> SSQQVWKLVIITEEILLKKVSKIIKEAGASGYTVLAAAGEGSRNVRSTGEPSVSHAYSNIKFEVLTASRELADQIQDKVVAKYFDDYSCITYISTVE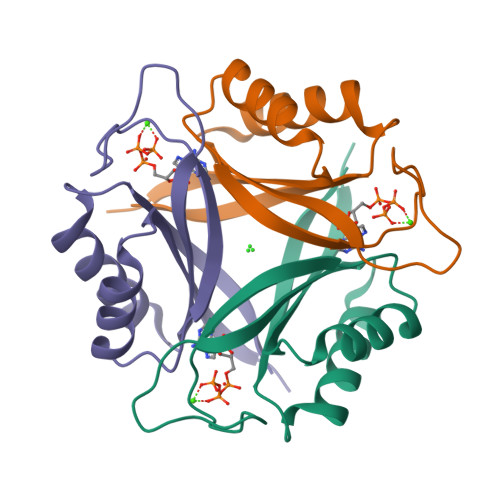ALRAHKF4-[8-methoxy-2-[(1-methylpyrazol-4-yl)amino]quinazolin-6-yl]phenol | C19 H17 N5 O2 | 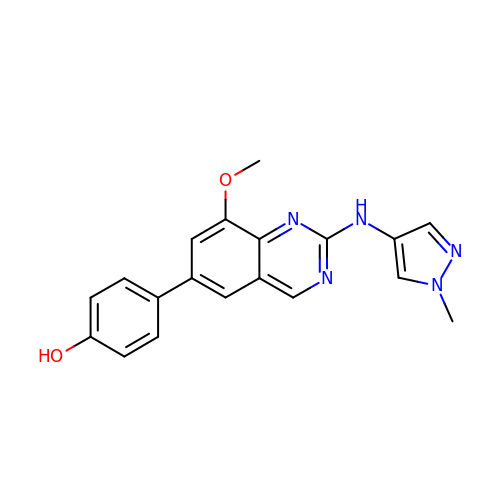GNVJDFYURAVLOR-UHFFFAOYSA-N> KEVC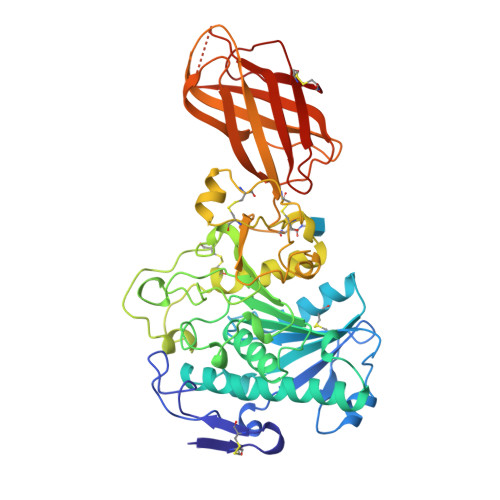YGHLGCFSNDKPWAGMLQRPLKIFPWSPEDIDTRFLLYTNENPNNYQKISATEPDTIKFSNFQLDRKTRFIVHGFIDKGEDGWLLDMCKKMFQVEKVNCICVDWRRGSRTEYTQASYNTRVVGAEIAFLVQVLSTEMGYSPENVHLIGHSLGAHVVGEAGRRLEGHVGRITGLDPAEPCFQGLPEEVRLDPSDAMFVDVIHTDSAPIIPYLGFGMSQKVGHLDFFPNGGKEMPGCQKNILSTIVDINGIWEGTQNFVACNHLRSYKYYASSILNPDGFLGYPCSSYEKFQQNDCFPCPEEGCPKMGHYADQFEGKTATVEQTVYLNTGDSGNFTRWRYKVSVTLSGAKKLSGYILVALYGNNGNSKQYEIFKGSLKPEARHVRDIDVDINVGEIQKVKFLWNNKVINLFRPTLGASQITVQSGVDGKEYNFCSSDTVREDVLQSLYPC>SMGRKVTVATCALNQWALDFEGNLQRILKSIEIAKNRGARYRLGPELEICGYGCWDHYYESDTLLHSFQVLAALLESPVTQDIICDVGMPVMHRNVRYNCRVIFLNRKILLIRPKMALANEGNYRELRWFTPWSRSRHTEEYFLPRMIQDLTKQETVPFGDAVLVTWDTCIGSEICEELWTPHSPHIDMGLDGVEIITNASGSHHVLRKANTRVDLVTMVTSKNGGIYLLANQKGCDGDRLYYDGCAMIAMNGSVFAQGSQFSLDDVEVLTATLDLEDVRSYRAEISSRNLAASRASPYPRVKVDFALSCHEDLLAPISEPIEWKYHSPEEEISLGPACWLWDFLRRSQQAGFLLPLSGGVDSAATACLIYSMCCQVCEAVRSGNEEVLADVRTIVNQISYTPQDPRDLCGRILTTCYMASKNSSQETCTRARELAQQIGSHHISLNIDPAVKAVMGIFSLVTGKSPLFAAHGGSSRENLALQNVQARIRMVLAYLFAQLSLWSRGVHGGLLVLGSANVDESLLGYLTKYDCSSADINPIGGISKTDLRAFVQFCIQRFQLPALQSILLAPATAELEPLADGQVSQTDEED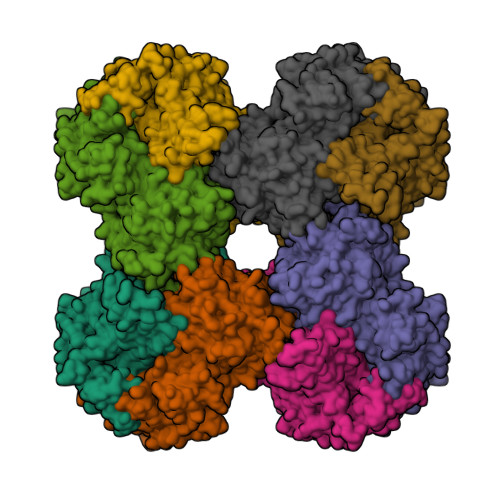MGMTYAELSVYGKLRKVAKMGPYSMFCKLLGMWRHICTPRQVADKVKRFFSKYSMNRHKMTTLTPAYHAENYSPEDNRFDLRPFLYNTSWPWQFRCIENQVLQLERAEPQSLDGVD[2x]> 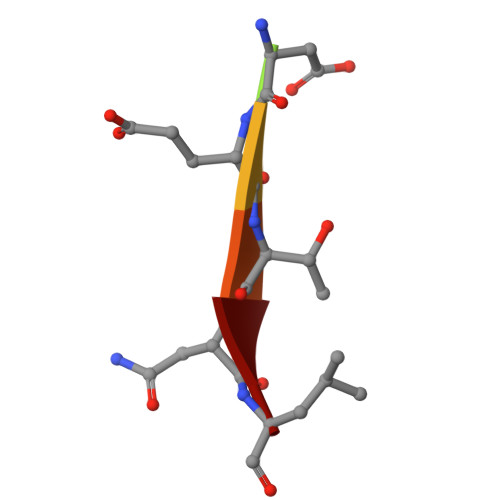AWDETNL>MIKMVIVVRSDIKMGKGKIAAQVAHAAVTLVVSIINSNNLRWKEWLNEWLHQGQPKIIVKVNSLDEIISRAKKAETMNLPFSIIEDAGKTQLEPGTITCLGIG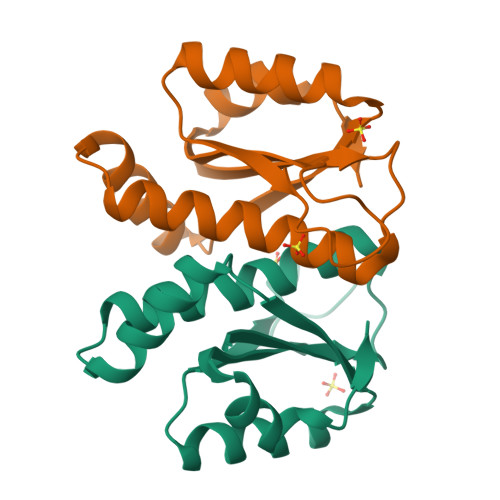PAPENLVDSITGDLKLL[4x]>[4x]MGP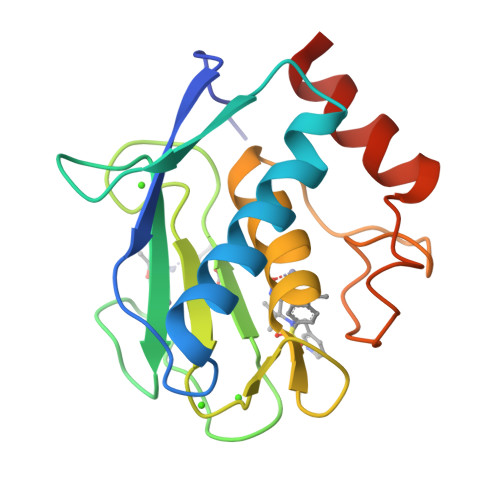VWRKHYITYRINNYTPDMNREDVDYAIRKAFQVWSNVTPLKFSKINTGMADILVVFARGAHGDFHAFDGKGGILAHAFGPGSGIGGDAHFDEDEFWTTHSGGTNLFLTAVHAIGHSLGLGHSSDPKAVMFPTYKYVDINTFRLSADDIRGIQSLYGHHHHH Bacillus phages use a communication system, termed “arbitrium,” to coordinate lysis-lysogeny decisions. Arbitrium communication is mediated by the production and secretion of a hexapeptide (AimP) during lytic cycle. Once internalized, AimP reduces the expression of the negative regulator of lysogeny, AimX, by binding to the transcription factor, AimR, promoting lysogeny. We have elucidated the crystal structures of AimR from the Bacillus subtilis SPbeta phage in its apo form, bound to its DNA operator and in complex with AimP.

The crystals of the AimR-AimP complex diffracted up to 2.3 Å resolution in space group P41212 containing two molecules of AimR in the asymmetric unit arranged as a dimer with one bound GMPRGA peptide per monomer. The peptide binds to the concave side of the channel formed by the TPR-like repeats of AimR. The peptide is bound in an extended conformation that allows contact with residues from all of the TPR motifs with the exception of TPR1. The peptide N-terminal amine is bound to Q299 and E300 side chains and to M296 main chain (TPR7), establishing hydrogen bonds and a salt bridge, while on the opposite end, the C-terminal carboxylate is salt bridged to R228 (TPR6) side chain. AimP R2 side chain, which is highly conserved among arbitrium peptides, interacts by hydrogen bonds with N206 (TPR5) and N329 (TPR8) and a salt bridge with D360 (TPR8 and TPR9 loop). The AimP-bound form presents a more compact conformation, reflected in a reduction of the superhelix pitch of ∼5 Å with respect to the DNA-bound form, and even bigger (∼11 Å) with respect to some apo forms. The closure movement induced by AimP binding (between 10° and 20° calculated with Dyndom [Hayward and Berendsen, 1998]) reduces the distance between the TPRN-ter and TPRC-ter subdomains, allowing new interactions between residues of both subdomains that stabilize the peptide-bound conformation. Superimposition of the two monomers present in AimR-AimP dimer showed that both subunits are almost identical. Comparison of AimP and DNA-bound structures confirms that the closed conformation induced by AimP reduces the distance between the DNA recognition helices. As a consequence, AimP fixes an AimR conformation unable to reach the two distant half sites of the AimR operator.

>MELIRIAMKKDLENDNSLMNKWATVAGLKNPNPLYDFLNHDGKTFNEFSSIVNIVKSQYPDREYELMKDYCLNLDVKTKAARSALEYADANMFFEIEDVLIDSMISCSNMKSKEYGKVYKIHRELSNSVITEFEAVKRLGKLNIKTPEMNSFSRLLLLYHYLSTGNFSPMAQLIKQIDLSEISENMYIRNTYQTRVHVLMSNIKLNENSLEECREYSKKALESTNILRFQVFSYLTIGNSLLFSNYELAQENFLKGLSISVQNENYNMIFQQALCFLNNVWRKENKWINFESDSIMDLQEQAHCFINFNENSKAKEVLDKLDLLVHNDNELAMHYYLKGRLEQNKACFYSSIEYFKKSNDKFLIRLPLLELQKMGENQKLLELLLL[2x];>[2x]GMPRGA>[2x]SNAMDFSDDNLIWLDLEMTGLDPERDRIIEIATIV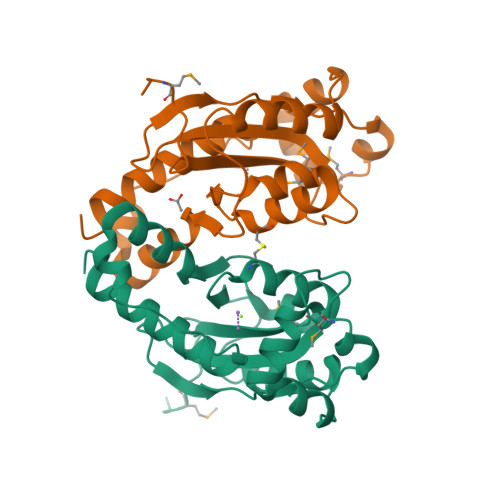TNSHLDILAEGPAFAIHQPDKLLTAMDNWNTSHHTASGLLERVKNSSVDEVEAETLTLAFLEKYVSAGKSPLCGNSVCQDRRFLSRYMPRLNQFFHYRHLDVTTLKILAQRWAPQIAAAHIKESQHLALQDIRDSIEELRYYRAHLLNLSK>MVEPSLVLYGAPYERAVEVLEETLRETGARYALLIDRKGFVLAHKEALWAPKPPPLDTLATLVAGNAAATQALAKLLGEARFQEEVHQGERMGLYVDEAGEHALLVLVFDETAPLGKVKLHGKRASEALARIAE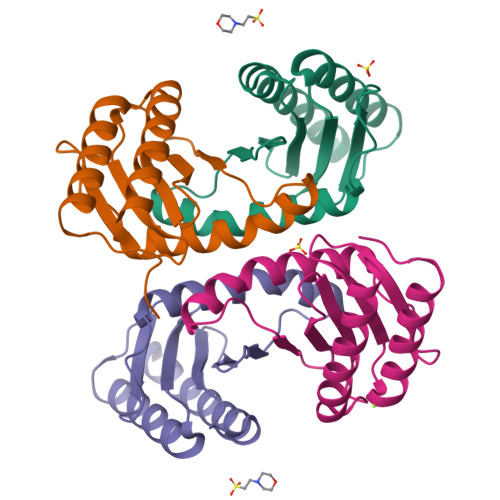EALANPPRLALDTEYREGAEALLDDLLRN[4x]> MKTSDANETEDHLESLICKVGEKSACSLESNLEGLAGVLEADLPNYKSKILRLLCTVARLLPEKLTIYTTLVGLLNARNYNFGGEFVEAMIRQLKESLKANNYNEAVYLVRFLSDLVNCHVIAAPSMVAMFENFVSVTQEEDVPQVRRDWYVYAFLSSLPWVGKELYEKKDAEMDRIFANTESYLKRRQKTHVPMLQVWTADKPHPQEEYLDCLWAQIQKLKKDRWQERHILRPYLAFDSILCEALQHNLPPFTPPPHTEDSVYPMPRVIFRMFDYTDDPEGPVMPGSHSVERFVIEENLHCIIKSHWKERKTCAAQLVSYPGKNKIPLNYHIVEVIFAELFQLPAPPHIDVMYTTLLIELCKLQPGSLPQVLAQATEMLYMRLDTMNTTCVDRFINWFSHHLSNFQFRWSWEDWSDCLSQDPESPKPKFVREVLEKCMRLSYHQRILDIVPPTFSALCPVNPTCIYKYGDESSNSLPGHSVALCLAVAFKSKATNDEIFSILKDVPNPNQDDDDDEGFSFNPLKIEVFVQTLLHLAAKSFSHSFSALAKFHEV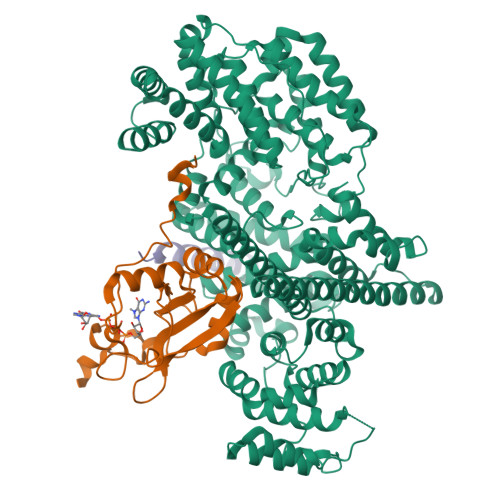FKTLAESDEGKLHVLRVMFEVWRNHPQMIAVLVDKMIRTQIVDCAAVANWIFSSELSRDFTRLFVWEILHSTIRKMNKHVLKIQKELEEAKEKLARQHKRRSDDDDRSSDRKDGVLEEQIERLQEKVESAQSEQKNLFLVIFQRFIMILTEHLVRCETDGTSVLTPWYKNCIERLQQIFLQHHQIIQQYMVTLENLLFTAELDPHILAVFQQFCALQA;> GAMSGGLLKALRSDSYVELSQYRDQHFRGDNEEQEKLLKKSCTLYVGNLSFYTTEEQIYELFSKSGDIKKIIMGLDKMKKTACGFCFVEYYSRADAENAMRYINGTRLDDRIIRTDWDAGFKEGRQYGRGRSGGQVRDEYRQDYDAGRGGYGKLAQNQ;> KKVDHRAPGAEEDDSELQRAWGALIKEKEQSRQKKSRLDNLPSLQIEVSRESSSGSEAES>MRILVVNVNTTASITETIAEQARAVASPGTEIVGLTPYFGAESVEGNFESYLAAIAVMDRVMAYDQPFDAVIQAGYGEHGREGLQELLNVPVVDITEAAASTAMFLGHAYSVVTTLDRTVPLIEDRLKLAGLYQRCASVRASGMAVLELEEDPVAAMEAIVRQAELAIREDKAEVICLGCGGMAGLDEQIRQRTGVPVVDGVTAAVT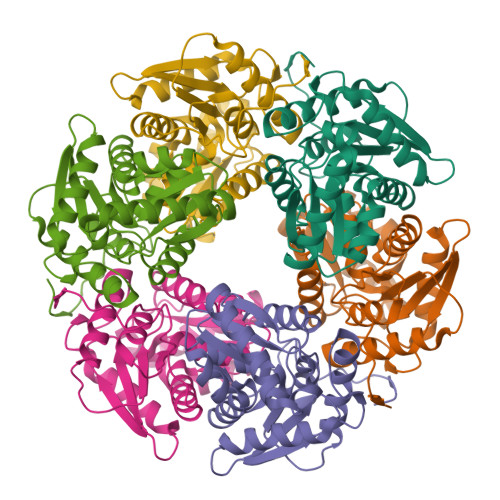IAESLVRLGLSTSKIRTYATPRPKKVIGWPGRLGR[6x]>MTARNPLEAQAWALLEAVYDPELGLDVVNLGLIYDLVVEPPRAYVRMTLTTPGCPLHDSLGEAVRQALSRLPGVEEVEVEVTFEPPWTLARLSEKARRL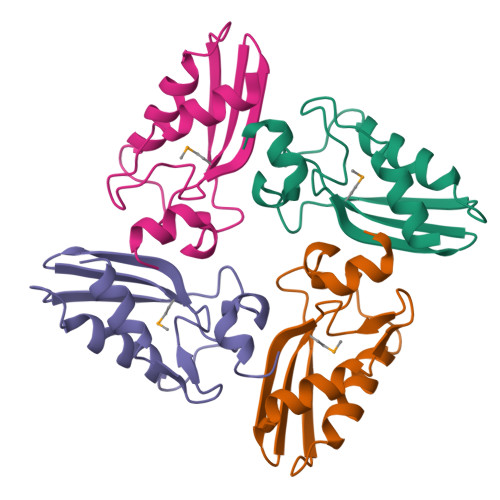LGWG[4x]>[2x]MQNITQSWFVQGMIKATTDAWLKGWDERNGGNLTLRLDDADIAP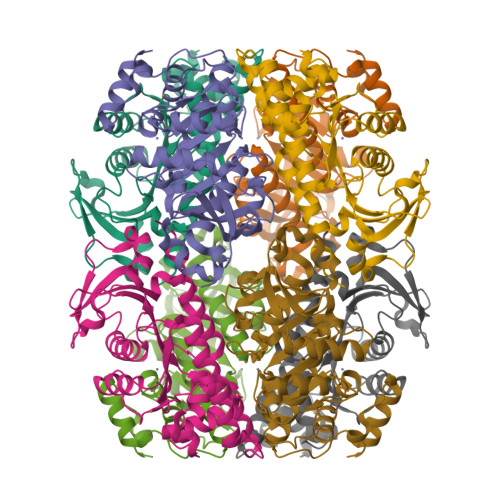YHDNFHQQPRYIPLSQPMPLLANTPFIVTGSGKFFRNVQLDPAFNLGIVKVDSDGAGYHILWGLTNEAVPTSELPAHFLSHCERIKATNGKDRVIMHCHATNLIALTYVLENDTAVFTRQLWEGSTECLVVFPDGVGILPWMVPGTDAIGQATAQEMQKHSLVLWPFHGVFGSGPTLDETFGLIDTAEKSAQVLVKVYSMGGMKQTISREELIALGKRFGVTPLASALAL> MPKLQEMMTIVSQREVASNIF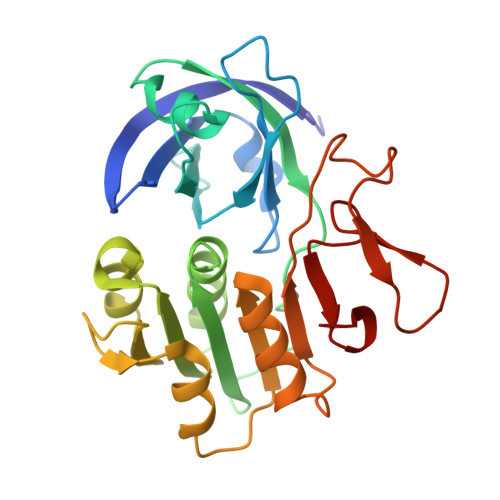EMVLKGELVEEMDLPGQFLHLAVPNASMLLRRPISISSWDKVAKTCTILYRIGDETSGTYEISKLQSGAKIDVMGPLGNGFPVDEVVSTDKILIVGGGIGVPPLYELAKQLEEKNCQMTILLGFASEKVKILEKEFAELKNVSLKIATDDGSYGTKGHVGMLMEEIDFEVDALYTCGAPAMLKAVAKKYEQLERLYISMESRMACGIGACYACVEHDKEDENHALKVCEDGPVFLGKQLLL>PVTTSFWRIATDARTYEADDLSGAGAKITGGRWNEVGVAIVYAASSRAMACLETVVHLNSGGLPLNRYLVEIEVPDEVLASAEVATPGNLPVGWDAEPAGRVSISFGSQWAQSQRTALLLVPSVIVPEETNLLINPAHPDAKGIKARKVRKWLYDPRMIR[2x];>VLGLAKLVGQLEDMVEESGETDGFDAPEWLSSWLRQPLPALGGVNPIDLLDTMEGQAVVSRALAQIQSGAFA[2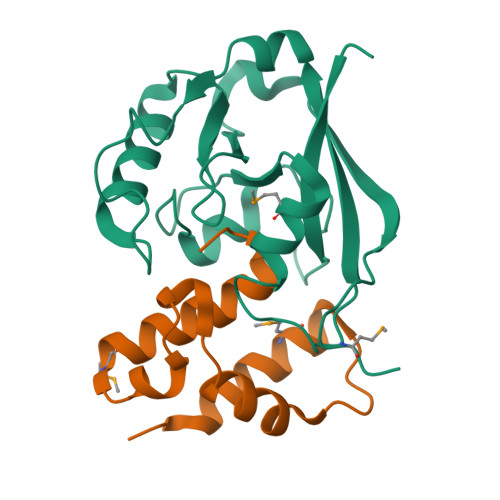x]>[8x]GEIRPTIGQQMETGDQRFGDLVFRQLA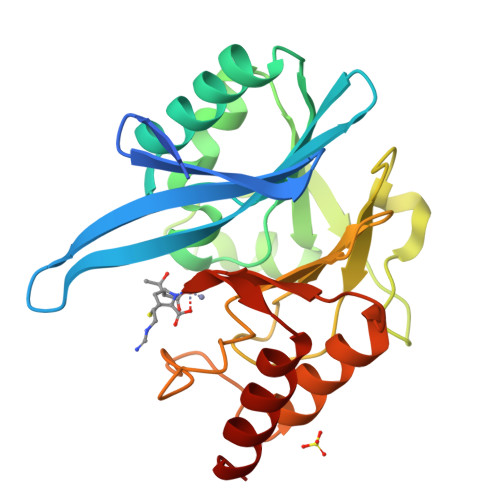PNVWQHTSYLDMPGFGAVASNGLIVRDGGRVLVVDTAWTDDQTAQILNWIKQEINLPVALAVVTHAHQDKMGGMDALHAAGIATYANALSNQLAPQEGMVAAQHSLTFAANGWVEPATAPNFGPLKVFYPGPGHTSDNITVGIDGTDIAFGGCLIKDSKAKSLGNLGDADTEHYAASARAFGAAFPKASMIVMSHSAPDSRAAITHTARMADKLR> GNMDSKAVEELSATE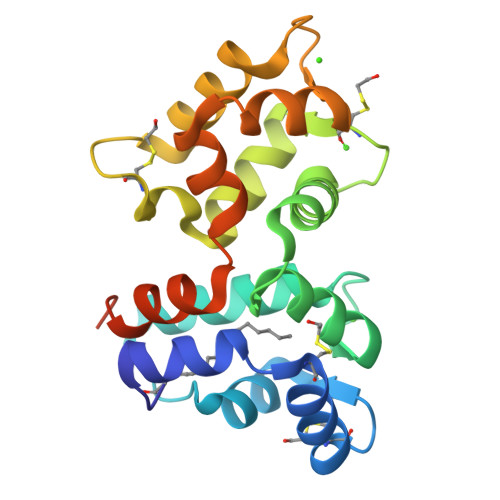CHQWYKKFMTECPSGQLTLYEFKQFFGLKNLSPSANKYVEQMFETFDFNKDGYIDFMEYVAALSLVLKGKVDQKLRWYFKLYDVDGNGCIDRGELLNIIKAIRAINRCNEAMTAEEFTNMVFDKIDINGDGELSLEEFMEGVQKDEVLLDILTRSLDLTHIVKLIQNDGKNPHAPEEAEEAAQ>[2x]MALAKRIDAALIVKDGRVVEGSNFENLRDSGDPVELGKFYSEIGIDELSFWDITASVEKRKTMLELVEKVAEQIDIPFTVGGGIHDFETASELILRGADKVEINTAAVENPSLITQIAQTFGSQAVVVYIAAKRVDGEFMVFTYSGTKNTGILLRDWVVEVEKRGAGEIVLGSIDRLGTKSGYDTEMIRFVRPLTTLPIIAHRGAGKMEHFLEAFLAGADAAKADSVFHFREIDVRELKEYLKKHGVNVRLEGLGSLEHHHHHH

Computational design of KE07 involved construction of a theozyme to catalyze the chemical reaction, which was then grafted into the scaffold of imidazole glycerol phosphate synthase (HisF) from Thermotoga maritima. Catalytically essential residues from the initial design include a base (Glu101) that facilitates C−H bond cleavage, an H-bond donor (Lys222) to stabilize the phenoxide intermediate, and a π-stacking residue (Trp50), which was designed to stabilize the transition state and favor substrate binding through interactions with the aromatic ring of the substrate. This initial KE07 design (Round 1; R1) catalyzes the cleavage of 5-nitrobenzisoxazole, with 103-fold rate acceleration over the noncatalyzed reaction and a turnover rate (kcat) of 0.018 s−1.

In contrast to the improvement in turnover rate across the first four rounds of mutagenesis, which was unambiguously the result of reduced activation energy due to changes to the local electrostatics of the active site via mutations within and near the active site, the catalytic efficiency of R5 and R6 is improved by more favorable collision frequency (the activation energy actually increases). Thus, the mechanism by which the remote mutations that appear in R5 and R6 increase activity is qualitatively different. This is mirrored in their location within the protein; in contrast to the initial mutations that affect the active site directly, the mutations in R5 (Val12Met) and R6 (Lys146Thr) are remote from the active site. We also solved a higher resolution structure (1.61 Å) of R6, in which the active site of both monomers in the asymmetric unit were observed to be fully in configuration B, with the imidazole ring (an analog of the benzisoxale substrate) of the histidine tag of a neighboring KE07 molecule in the crystal lattice bound to the active site. The anomalous KIEs observed in R5−R6 correlate with the increased sampling of the alternative active site configurations.> MGEDYLKLLEEALKIAREVLENYPLTPVMRAAARAIIEAVKMAKKYGDEELIKLVVEAARLLRQAAKQG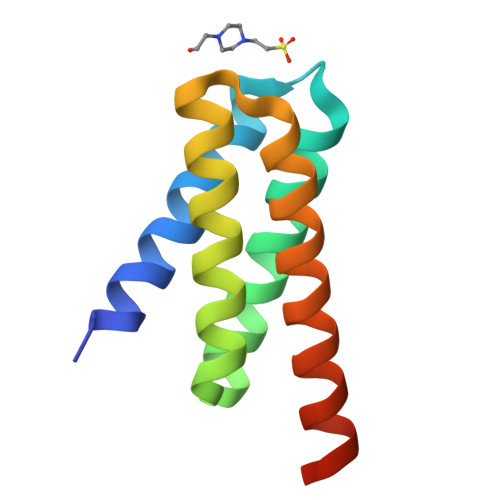DLELARQALAAARQALAFARRVAGLEHHHHHH UGT74F1 and UGT74F2 are the enzymes responsible for the in vivo glucosylation of SA in A. thaliana. In UGT74F1, glucose is transferred to the hydroxyl of SA, creating a glucoside; in UGT74F2, glucose is transferred to the carboxylate group of SA to create a glucose ester. UGT74F2 exhibits the GT-B fold with ligands bound in the cleft between the two domains –the N-terminal domain is comprised of residues 1–245, while 246–449 make up the C-terminal domain. UDP and SA interact primarily with residues in the C- and N-terminal domain, respectively.

We crystalized UGT74F2T15S and UGT74F2T15A in complex with UDP and SA or UDP and 2-BA. As the findings with both mutants were identical, we will present further the structures of UGT74F2T15S. The UDP and SA complex structure of this mutant is very similar to that of the wild-type enzyme, with an overall RMSD of 1.4 Å2. In contrast to the wild type enzyme, the omit map for SA in the binding pocket of UGT74F2T15S does not have clear electron density for the 2-hydroxyl of SA, despite the higher resolution of the latter structure. In contrast, UGT74F2T15A and UGT74F2T15S form both SGE and SAG; UGT74F2T15A has wild-type activity for SGE formation, better than UGT74F2T15S, and both mutants form about 5-fold more SAG than the wild-type. Therefore, we propose that SA binds to UGT74F2 primarily in the conformation described for the UDP/SA complex (i.e. carboxyl group of SA interacting with His 18 and Thr 15) but binds to UGT74F1 primarily in the conformation modeled on the basis of 2-BA in the 2-BA/UDP complexes of UGT74F2 wild-type or T15S (i.e. SA hydroxyl interacting with His 18 and SA carboxyl interacting with Thr 365). This explains why UGT74F1S15T and UGT74F2T365A behave like wild-type enzymes (no carboxyl group from SA to interact with) while UGT74F2T15S and UGT74F1T365A impact product specificity (both mutations affect interaction with SA carboxyl); the latter mutants can accommodate both binding modes of SA. Therefore, impairing the recognition of SA carboxyl group in each enzyme decreases the product specificity.

>MEHKRGHVLAVPYPSQGHITPFRQFCKRLHFKGLKTTLALTTFVFNSINPDLSGPISIATISDGYDHGGFETADSIDDYLKDFKTSGSKTIADIIQKHQTSDNPITCIVYDAFLPWALDVAREFGLVATPFFTQPCAVNYVYYLSYINNGSLQLPIEELPFLELQDLPSFFSVSGSYPAYFEMVLQQFINFEKADFVLVNSFQELELHENELWSKACPVLTIGPTIPSIYLDQRIKSDTGYDLNLFESKDDSFCINWLDTRPQGSVVYVAFGSMAQLTNVQMEELASAVSNFSFLWVVRSSEEEKLPSGFLETVNKEKSLVLKWSPQLQVLSNKAIGCFLTHCGWNSTMEALTFGVPMVAMPQWTDQPMNAKYIQDVWKAGVRVKTEKESGIAKREEIEFSIKEVMEGERSKEMKKNVKKWRDLAVKSLNEGGSTDTNIDTFVSRVQSK[2x]>IPLARTVRCNCI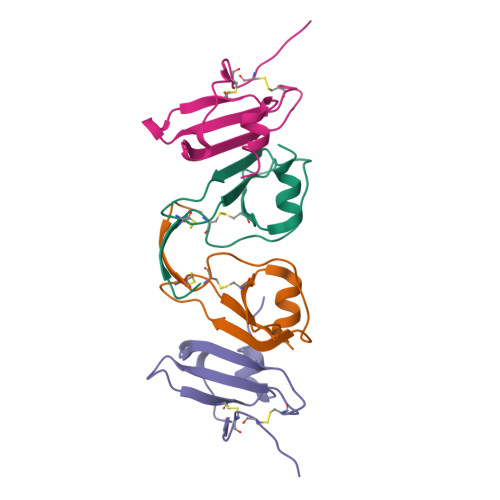HIDDGPVRMRAIGKLEIIPASLSCPRVEIIATMKKNDEQRCLNPESKTIKNLMKAF[4x]>[6x]HMFEIKKICCIGAGYVGGPTCSVIAHMCPEIRVTVVDVNESRINAWNSPTLPIYEPGLKEVVESCRGKNLFFSTNIDDAIKEADLVFISVNTPTKTYGMGKGRAADLKYIEACARRIVQNSNGYKIVTEKSTVPVRAAESIRRIFDANTKPNLNLQVLSNPEFLAEGTAIKDLKNPDRVLIGGDETPEGQRAVQALCAVYEHWVPREKILTTNTWSSELS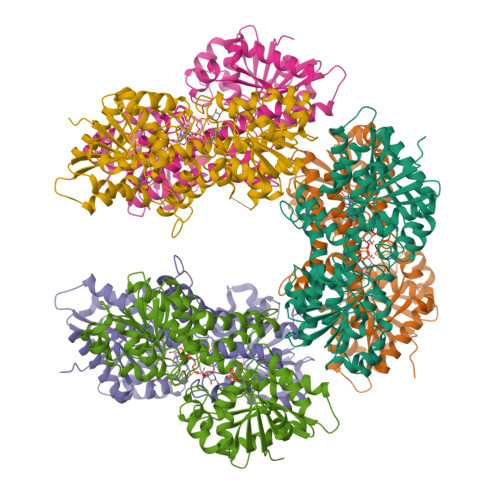KLAANAFLAQRISSINSISALCEATGADVEEVATAIGMDQRIGNKFLKASVGFGGSCFQKDVLNLVYLCEALNLPEVARYWQQVIDMNDYQRRRFASRIIDSLFNTVTDKKIAILGFAFKKDTGDTRESSSIYISKYLMDEGAHLHIYDPKVPREQIVVDLSHPGVSEDDQVSRLVTISKDPYEACDGAHAVVICTEWDMFKELDYERIHKKMLKPAFIFDGRRVLDGLHNELQTIGFQIETIGKKVSSKRIPYAPSGEIPKFSLQDPPNKKPKV>[7x]TEISFTNKNDTREIVDEVVENAFSSVCSTMGPNGNYVVINQLNSPKVTKDGVSVARALDFNEARRNMIAKIITEPSIKTDAEVGDGTTTTVFITYHLYQKFKDAMSFANTRYLDTLIKQVLQYIGTLIQPGEIESEMFRNMLLTSSNYEEEIVDKILDIYREHKNPNIHLEKSPMLPADEVKMTKEIYFEGSFPIETQVPANGAYVVGPEKVGVVLIDGSIRAYPTQLINALLNRFIDNPVVLMARNFEPEVIAAINNENQRLGTSRIFAYKVNAAGLLGAGTI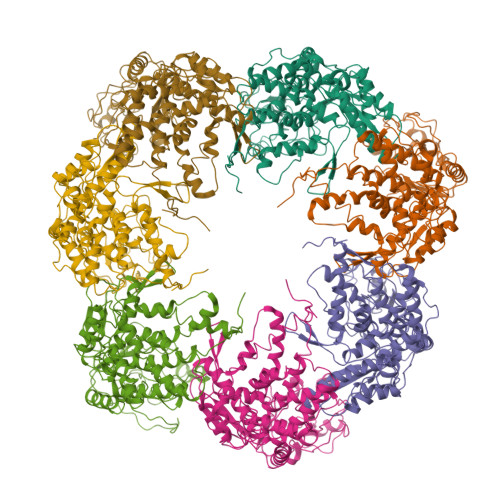DDLGRLLNIGPVFDVNSVDPALVKYNDVTLWLGRKGILLDKSIEEVESRADSILEGLDNRYEALGIIERQTPIGRELNRRIGRLRANNVTIKVTGVTVSDASERWARYEDVMKAARTGQQFGVIPGIGYGYLMASKWLEANVPQQSDEKLEKCRIGLIEVLRAQYEHLTGHDGSAENPIFIDLVTGQESDTPMNVYDNAAATMIALEGAWQTAKTLGKISNVMGRSNTNYA5-bromanyl-2-[(phenylmethyl)sulfonylamino]benzoic acid | C14 H12 Br N O4 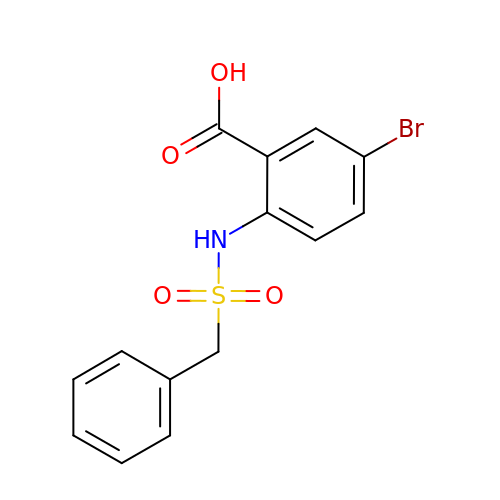S | RQMLGQUAXPPRSN-UHFFFAOYSA-N>VLSSLRMAAILDDQTVCGRGERLALALAREQINGIIEVPAKARVEVDIFELQRDSQYETTDTMCQILPKGVVSVLGPSSSPASASTVSHICGEKEIPHIKVGPEETPRLQYLRFASVSLYPSNEDVSLAVSRILKSFNYPSASLICAKAECLLRLEELVRGFLISKETLSVRMLDDSRDPTPLLKEIRDDKVSTIIIDANASISHLVLRKASELGMTSAF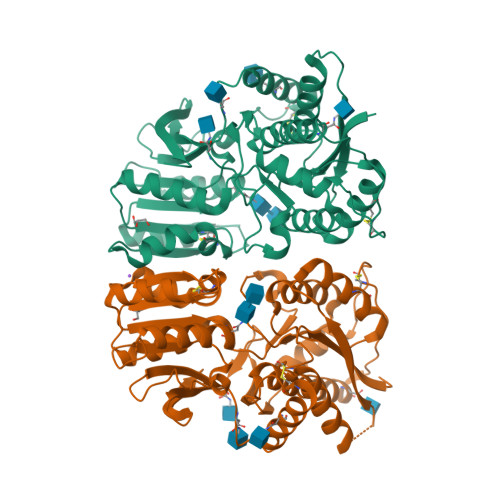YKYILTTMDFPILHLDGIVEDSSNILGFSMFNTSHPFYPEFVRSLNMSWRENCEASTYPGPALSAALMFDAVHVVVSAVRELNRSQEIGVKPLACTSANIWPHGTSLMNYLRMVEYDGLTGRVEFNSKGQRTNYTLRILEKSRQGHREIGVWYSNRTLAMNATTLDILELVPR[2x]(S)-4-(4-(3-(3-CARBAMIMIDOYLPHENYL)-2-(2,4,6-TRIISOPROPYLPHENYLSULFONAMIDO)PROPANOYL)PIPERAZINE-1-CARBONYL)PIPERIDINE-1-CARBOXIMIDAMIDE 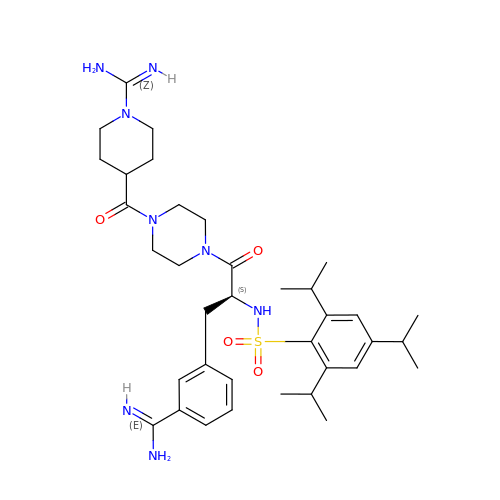| C36 H54 N8 O4 S | KSEVHDWJTMMENT-HKBQPEDESA-N>MSLTKYTIGV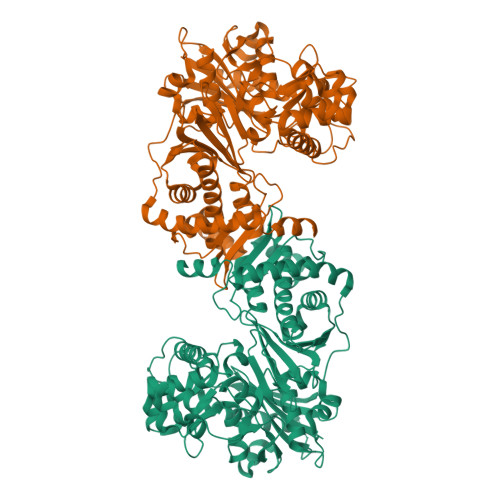DYGTESGRAVLIDLSNGQELADHVTPYRHGVIDQYLPNTNIKLGHEWALQHPLDYVEVLTTSVPAVMKESGVDADDVIGIGVDFTACTMLPVDEEGQPLCLLAQYKDNPHSWVKLWKHHAAQDKANAINEMAEKRGEAFLPRYGGKISSEWMIAKVWQILDEAEDVYNRTDQFLEATDWIVSQMTGKIVKNSCTAGYKAIWHKREGYPSNEFFKALDPRLEHLTTTKLRGDIVPLGERAGGLLPEMAEKMGLNPGIAVAVGNVDAHAAVPAVGVTTPGKLVMAMGTSICHMLLGEKEQEVEGMCGVVEDGIIPGYLGYEAGQSAVGDIFAWFVKHGVSAATFDEAQEKGVNVHALLEEKASQLRPGESGLLALDWWNGNRSILVDTELSGMLLGYTLQTKPEEIYRALLEATAFGTRAIVDAFHGRGVEVHELYACGGLPQKNHLLMQIFADVTNREIKVAASKQTPALGAAMFASVAAGSEVGGYDSIEEAAKKMGRVKDETFKPIPEHVAIYEKLYQEYVTLHDYFGRGANDVMKRLKALKSIQHRPSSLLTEGHHHHHH[4x]>[2x]NAAEVIVYEHVNFGG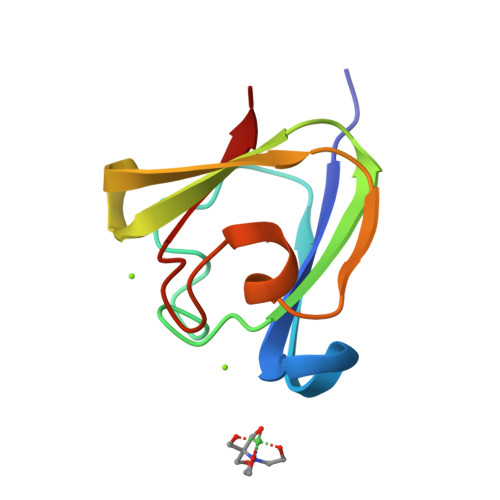KSFDATSDQPGAGDNLNDKISSIKVKSGTWRFYEYINYGGRYWDLGPGEYSSVESAGIPDNSISSFRQI>GPDSASRISPGQINQVRPKLPLLKILHAAGAQGEMFTVKEVMHYLGQYIMVKQLYDQQEQHMVYCGGDLLGELLGRQSFSVKDPSPLYDMLRK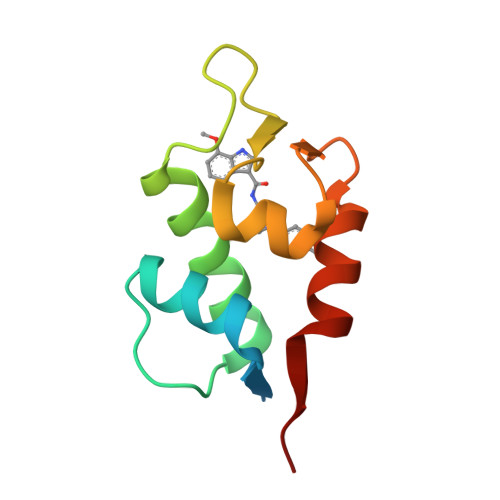NLVTLAT[2x]> MARKVTTRWKITGTLIAETPLHIGGVGGDADTDLALAVNGAGEYYVPGTSLAGALRGWMTQLLNNDESQIKDLWGDHLDAKRGASFVIVDDAVIHIPNNADVEIREG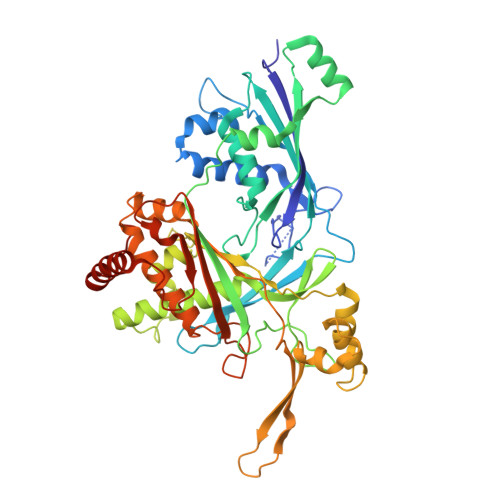VGIDRHFGTAANGFKYSRAVIPKGSKFKLPLTFDSQDDGLPNALIQLLCALEAGDIRLGAAKTRGLGRIKLDDLKLKSFALDKPEGIFSALLDQGKKLDWNQLKANVTYQSPPYLGISITWNPKDPVMVKAEGDGLAIDILPLVSQVGSDVRFVIPGSSIKGILRTQAERIIRTICQSNGSEKNFLEQLRINLVNELFGSASLSQKQNGKDIDLGKIGALAVNDCFSSLSMTPDQWKAVENATEMTGNLQPALKQATGYPNNISQAYKVLQPAMHVAVDRWTGGAAEGMLYSVLEPIGVTWEPIQVHLDIARLKNYYHGKEEKLKPAIALLLLVLRDLANKKIPVGYGTNRGMGTITVSQITLNGKALPTELEPLNKTMTCPNLTDLDEAFRQDLSTAWKEWIADPIDLCQQEAA>[2x]MPYVEIIEQPKQRGM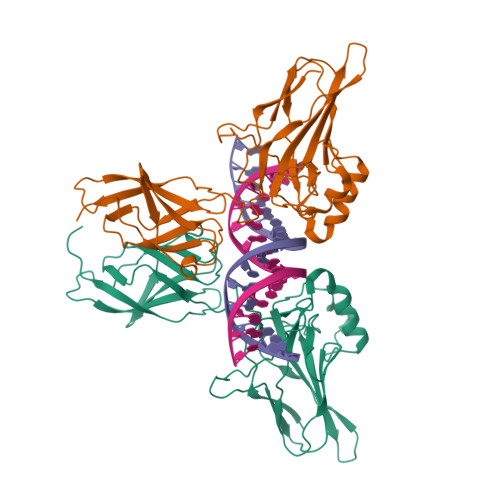RFRYKCEGRSAGSIPGERSTDTTKTHPTIKINGYTGPGTVRISLVTKDPPHRPHPHELVGKDCRDGYYEADLCPDRSIHSFQNLGIQCVKKRDLEQAISQRIQTNNNPFHVPIEEQRGDYDLNAVRLCFQVTVRDPAGRPLLLTPVLSHPIFDNRAPNTAELKICRVNRNSGSCLGGDEIFLLCDKVQKEDIEVYFTGPGWEARGSFSQADVHRQVAIVFRTPPYADPSLQAPVRVSMQLRRPSDRELSEPMEFQYLPDTDDRHRIEEKRKR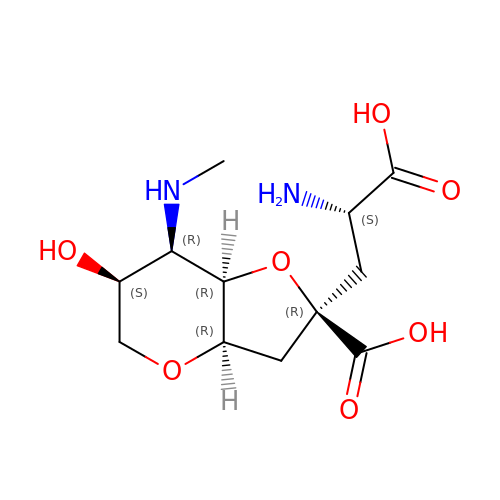(2R,3aR,6S,7R,7aR)-2-[(2S)-2-amino-2-carboxyethyl]-6-hydroxy-7-(methylamino)hexahydro-2H-furo[3,2-b]pyran-2-carboxylic acid | C12 H20 N2 O7 | YUSZFKPLFIQTGF-FDNSHYBFSA-N>MRGSFANDATFEIKKCDLHRLEEGPPVTTVLTREDGLKYYRMMQTVRRMELKADQLYKQKIIRGFCHLCDGQEACCVGLEAGINPTDHLITAYRAHGFTFTRGLSVREILAELTGRKGGCAKGKGGSMHMYAKNFYGGNGIMGAQVPLGAGIALACKYNGKDEVCLTLYGDGAANQGQIFEAYNMAALWKLPCIFICENNRYGMGTSVERAAASTDYYKRGDFIPGLRVDGMDILCVREATRFAAAYCRSGKGPILMELQTYRYHGHSMSDPGVSYRTREEIQEVRSKSDPIMLLKDRMVNSNLASVEELKEIDVEVRKEIEDAAQFATADPEPPLEELGYHIYSSDPPFEVRGANQWIKFKSVS[4x];>GSLQVTVRDAINQGMDEELERDEKVFLLGEEVAQYDGAYKVSRGLWKKYGDKRIIDTPISEMGFAGIAVGAAMAGLRPICEFMTFNFSMQAIDQVINSAAKTYYMSGGLQPVPIVFRGPNGASAGVAAQHSQCFAAWYGHCPGLKVVSPWNSEDAKGLIKSAIRDNNPVVVLENELMYGVPFEFPPEAQSKDF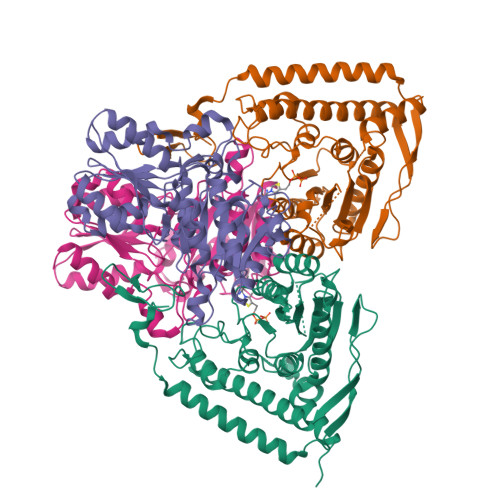LIPIGKAKIERQGTHITVVSHSRPVGHCLEAAAVLSKEGVECEVINMRTIRPMDMETIEASVMKTNHLVTVEGGWPQFGVGAEICARIMEGPAFNFLDAPAVRVTGADVPMPYAKILEDNSIPQVKDIIFAIKKTLNI[4x]>MSDWSGSVPANAENGKSTGLILKQGDTISVVAHGWVKYGRDNVEWAAPDGPVPNNPQPSSIATLVAKIANKKFAIGNGVLHKTVPV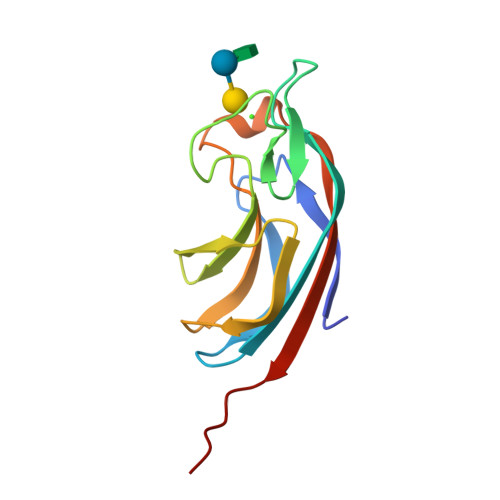DGELILLFNDVPGTFGDNSGEFQVEVIIESRYSPLK[8x]>MGHHHHHHGTKQEKTALNMARFIQNQTQTLLEKLNELDADEQADIAESLHDHADELYRSALAR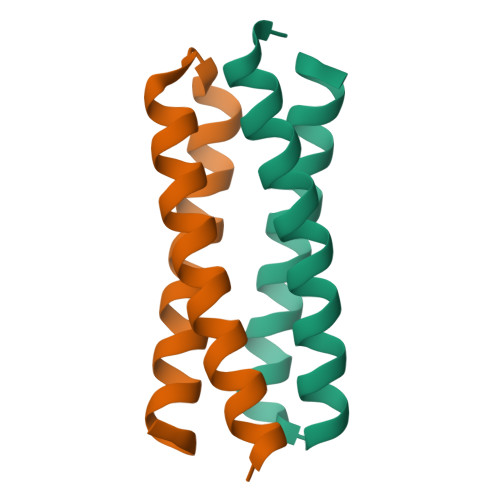WG[2x]> MKLVIEG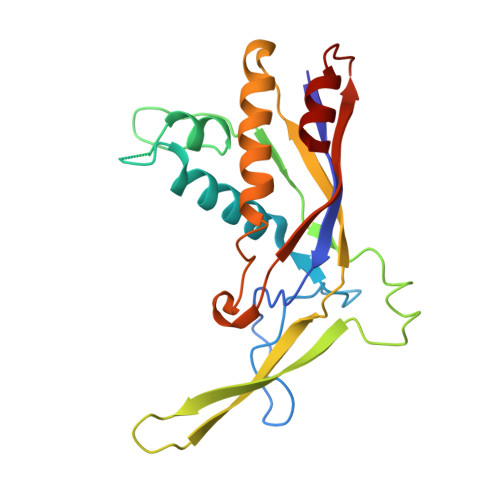TIVLKTGMHIGGSSDFSAIGAVASPVVRDTLTRLPLIPGSSLKGKMRYLLAKELNNGILLNEPNNDQDEILRLFGSSEKDKIRRARLKFNDIKLSNLAELETFNVSSTEVKFENTINRKTAVANPRQIERVIAGSKFDFEIFYNLDDIKEVEKDFENIKQGFDLLEFDYLGGHGTRGSGRIAFENLSVITAVGNFEKINTLNEILGA> MKSPEELKGIFEKYAAKEGDPNQLSKEELKLLLQTEFPSLLKGP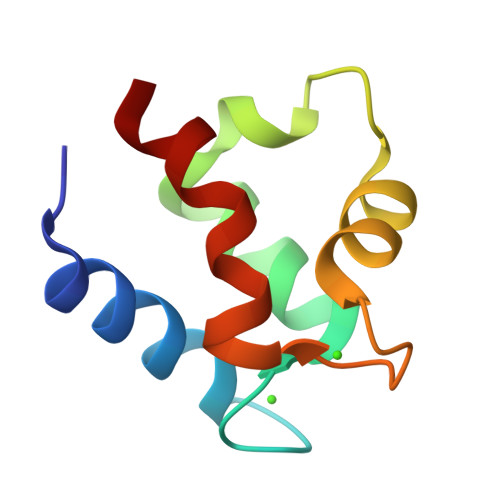STLDELFEELDKNGDGEVSFEEFQVLVKKISQ>[4x]MQFRSIIRIVGLLLALFSVTMLAPALVALLYRDGAGVPFVTTFFVLLFCGAMCWFPNRRHKHELKSRDGFLIVVLFWTVLGSAGSLPFLIADNPNISVTDAFFESFSALTTTGATVIVGLDELPKAILFYRQFLQWFGGMGIIVLAVAILPVLGIGGMQLYRAEIPGPVKDTKMTPRIAE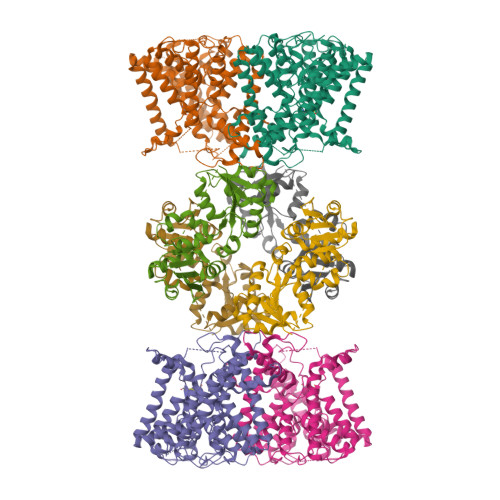TAKALWYIYLSLTIACAVAFWLAGMTPFDAISHSFSTIAIGGFSTHDASMGYFDSYAINLITVVFLLISACNFTLHFAAFASGGVHPKYYWKDPEFRAFIFIQVLLFLVCFLLLLKHHSYTSPYDAFDQALFQTVSISTTAGFTTTGFADWPLFLPVLLLFSSFIGGCAGSTGGGMKVIRILLLTLQGARELKRLVHPRAVYTIKVGGSALPQRVVDAVWGFFSAYALVFVVCMLGLIATGMDELSAFSAVAATLNNLGPGLGEVALHFGDVNDKAKWVLIVSMLFGRLEIFTLLILLTPTFWRS;>MKIIILGAGQVGGTLAENLVGENNDITIVDNNADRLRELQDKYDLRVVNGHASHPDVLHEAGAQDADMLVAVTNTDETNMAACQVAFTLFNTPNRVARIRSPEYLAEKEALFKSGAIPVDHLIAPEELVTSYIERLIQYPGALQVVSFAEQKVSLVAVKAYYGGPLVGNALSALREHMPHIDTRVAAIFRQGRPIRPQGTTIIEADDEVFFVAASNHIRSVMSELQRLEKPYRRIMIVGGGNIGASLAKRLEQTYSVKLIERDYQRAEKLSEQLENTIVFCGDAADQELLTEENIDQVDVFIALTNEDETNIMSAMLAKRMGAKKVMVLIQRGAYVDLVQGGVIDVAISPQQATISALLTHVRRADIVNVSSLRRGAAEAIEAVAHGDETTSKVVGRAIGDIKLPPGTTIGAVVRGEEVLIAHDRTVIEQDDHVVMFLVDKKYVPDVEALFQPSPFFL[4x]> MIYLKSFERNIRLINMKVVYDDVRVLKDIIQALARLVDEAVLKFKQDSVELVALDRAHISLISVNLPREMFKEYDVNDEFKFGFNTQYLMKILKVAKRKEAIEIASE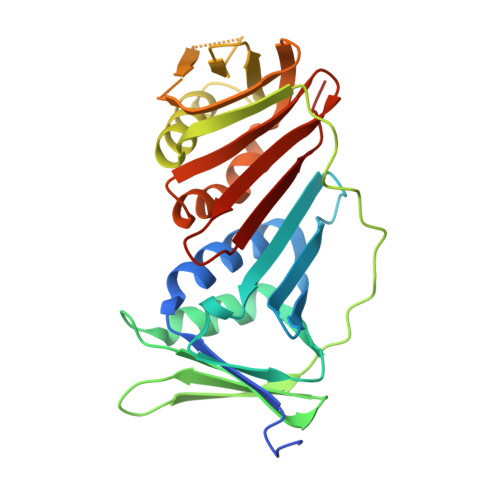SPDSVIINIIGSTNREFNVRNLEVSEQEIPEINLQFDISATISSDGFKSAISEVSTVTDNVVVEGHEDRILIKAEGESEVEVEFSKDTGGLQDLEFSKESKNSYSAEYLDDVLSLTKLSDYVKISFGNQKPLQLFFNMEGGGKVTYLLAPKV> VPDVMVVGEP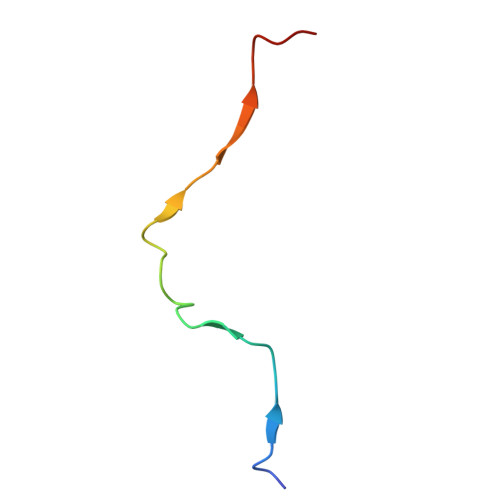TLMGGEFGDEDERLITRLENTQFDA>MSDTDIQDQQPD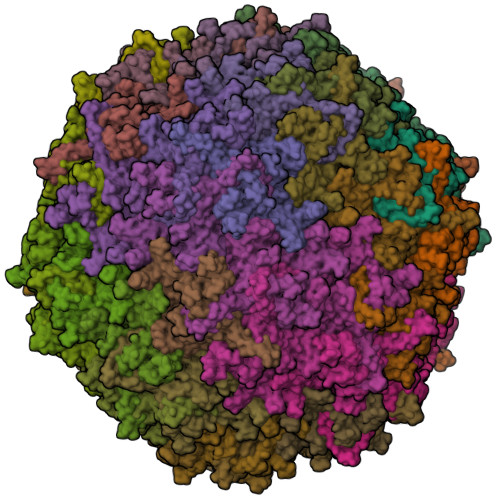TVDAPQNTSGGGTGSIGGGKGSGVGISTGGWVGGSHFSDKYVVTKNTRQFITTIQNGHLYKTEAIETTNQSGKSQRCVTTPWTYFNFNQYSCHFSPQDWQRLTNEYKRFRPKAMQVKIYNLQIKQILSNGADTTYNNDLTAGVHIFCDGEHAYPNASHPWDEDVMPDLPYKTWKLFQYGYIPIENELADLDGNAAGGNATEKALLYQMPFFLLENSDHQVLRTGESTEFTFNFDCEWVNNERAYIPPGLMFNPKVPTRRVQYIRQNGSTAASTGRIQPYSKPTSWMTGPGLLSAQRVGPQSSDTAPFMVCTNPEGTHINTGAAGFGSGFDPPSGCLAPTNLEYKLQWYQTPEGTGNNGNIIANPSLSMLRDQLLYKGNQTTYNLVGDIWMFPNQVWDRFPITRENPIWCKKPRADKHTIMDPFDGSIAMDHPPGTIFIKMAKIPVPTASNADSYLNIYCTGQVSCEIVWEVERYATKNWRPERRHTALGMSLGGESNYTPTYHVDPTGAYIQPTSYDQCMPVKTNINKVL[60x]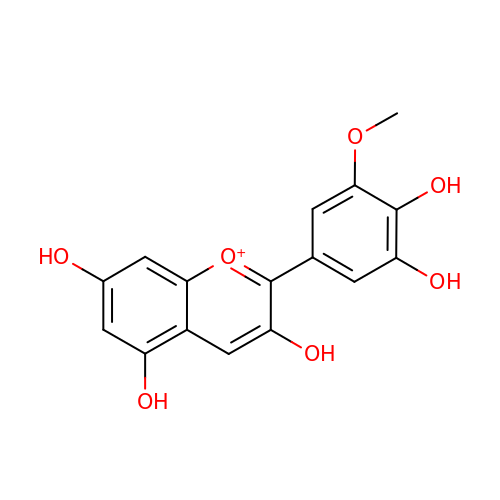2-(3,4-dihydroxy-5-methoxyphenyl)-3,5,7-trihydroxychromenium | C16 H13 O7 | AFOLOMGWVXKIQL-UHFFFAOYSA-O> MADEERLKEFKEANKIVFDPNTRQVWENQNRDGTKPATTFQSEEDIKRAAPESEKDTSATSGIVPTLQNIVATVT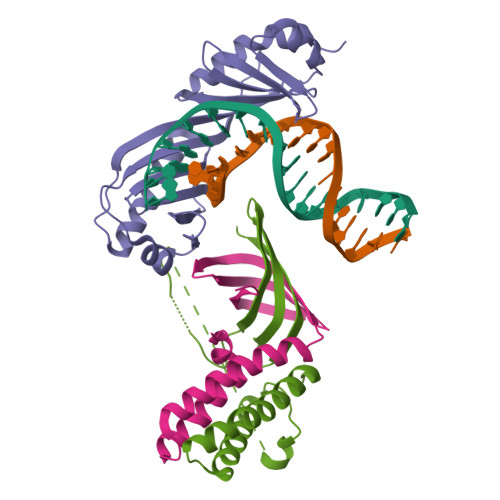LGCRLDLKTVALHARNAEYNPKRFAAVIMRIREPKTTALIFASGKMVVTGAKSEDDSKLASRKYARIIQKIGFAAKFTDFKIQNIVGSCDVKFPIRLEGLAFSHGTFSSYEPELFPGLIYRMVKPKIVLLIFVSGKIVLTGAKQREEIYQAFEAIYPVLSEFRKM;> MAVPGYYELYRRSTIGNSLVDALDTLISDGRIEASLAMRVLETFDKVVAETLKDNTQSKLTVKGNLDTYGFCDDVWTFIVKNCQVTVEDSHRDASQNGSGDSQSVISVDKLRIVACNSKKSE;> MSNAEASRVYEIIVESVVNEVREDFENAGIDEQTLQDLKNIWQKKLTETKVTTFSWDNQFNEGNINGVQNDLNFNLATPGVNSSEFNIKEENTGNEGLILPNINSNNNIPHSGETNINTNTVEATNNSGATLNTNTSGNTNADVTSQPKIEVKPEIELTINNANITTVENIDDESEKKDDEEKEEDVEKTRKEKEQIEQVKLQAKKEKRSALLDTDEVGSELDDSDDDYLISEGEEDGPDENLMLCLYDKVTRTKARWKCSLKDGVVTINRNDYTFQKAQVEAEWV> DNPPWAKPFELLVSFLNTPKYGTFDPTPVVPVFFPFWFGMIVGDIGYALLFYLVGRWLSGYVKRNEPLVIDLFALKLKPQVIGKLVHILNWMVFWTVVWGVIYGEFFGTFLEHLGVFGTPEHPGLIPILIHRIDTAKTANLLILLSVAFGVVLVFFGLALRAYLGLKHRHMAHFWEGVGYLGGLVGVLALAASYLGNLQAGWLQGLMYLGFGVFLLAVLMSRIWLMIPEIFTQAGHILSHIRIYAVGAAGGILAGLLTDVGFALAERLGLLGVLLGLLVAGVLHLLILLLTTLGHMLQPIRLLWVEFFTKFGF;>SGGL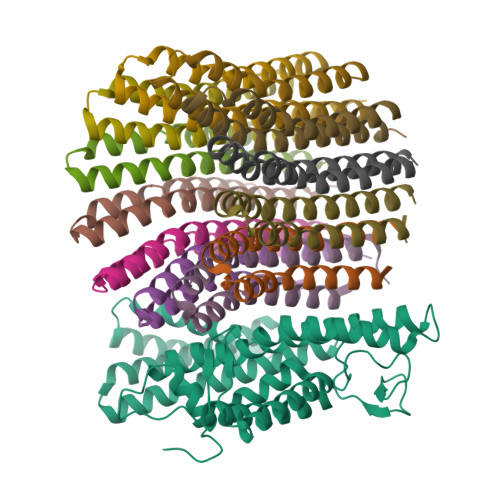DRGLIAVGMGLAVGLAALGTGVAQARIGAAGVGAIAEDRSNFGTALIFLLLPETLVIFGLLIAFILNGRL[12x]>SNAMDSRFLPATAFIDPEGRNRNEVERLVQQVVDLILAKLTGAAERPPMPETVDLPGPITIPEAAATEATLLQAIRDMVDGSMNPANPGYIGHMDPMPATMAILGDLVAAAVNNNMLSLEMSPSFSRLETLLLRAIAGLFGLGEQAGGVLTSGGSLANLQALAVARNVAFDSVEPGITGLAQRPVIFASEAAHTSLQKAAMLLGLGTAAVIPVRATADSRMDPEDLRARIDQARGAGQHPFCVVATAGTTTTGNIDPLAEIGAIAREHGLWFHVDAAYGGALVFSERHRWRLAGIEQADSITFNPQKWLYVAKTCAMVLFRDAGVLERAFRIPAPYMRATDGFINLGEIGVQGTRHADVVKLWLTLQHIGQQGYARLIDDGYRLAERVVE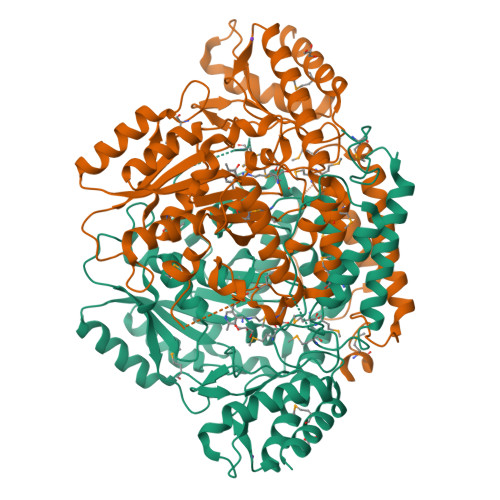GVRQRPFLRLAGEIDTNIVCFRGEPDWLPAERWDDWNAALQALLLREGKIFLSLPVYRGGRWLRAVLLNPYTTDAVIDAMFKQIDRFAGRERGQER[4x]> MEKLEALKISSMRPRSNILDRPLSKGKTEVSQSIVALLFSEIVQYSQS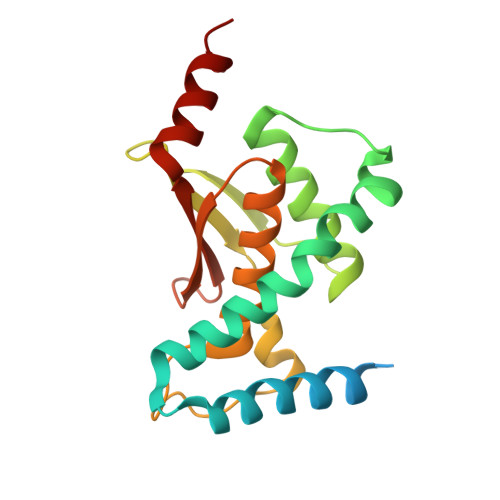RVFTVPELQTRLHDLGQDVGTRIIDLYFVRERSSKRETKLTQMLLFVKTTVWKNLFGKEAEKLEHANDDERTYYIIEKEPLVNTFISVPKDKGSLNCANFTAGIVEAVLTNCGFPCKVTAHWHKGTTYMVKFEDFVIARDKQMEEK>AAMIZTZKYHNGZKKYTPFSZAEMTRRZBRLRAWMAKSBIDAVLFTSYHNINYYSGWLYCYFGRKYAZVIBZVKAVTISKGIDGGMPWRRSFGBNIVYTDWKRDNFYSAVKKLVKGAKZIGIEHDHVTLBHRRZLZKALPGTEFVDVGZPVMWZRVIKSSEEZBLIRZGARISDIGGAATAAAISAGVPEYEVAIATTBAMVRZIARBFPYVELMDTWIWFQSGINTDGAHNPVTBRVVZRGDILSLNCFPMIFGYYTALERTLFLZZVBDASLZIWZKNTAVHRRGLZLIKPGARCKDIASELNBMYRZWDLLRYRTFGYGHSFGVLBHYYGREAGVELREDIZTVLEPGMVVSMEPMVMBPEGEPGAGGYREHDILV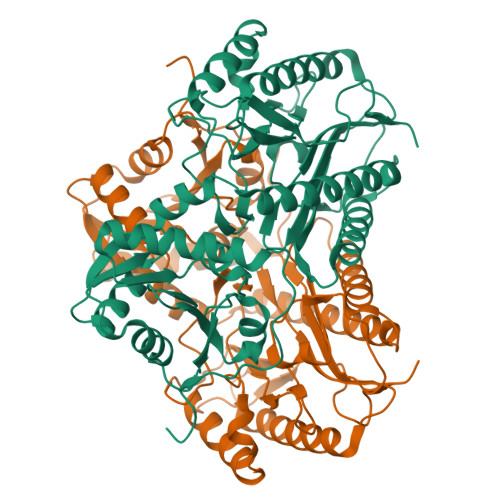IKENBTENITGFPFGPEHNIIKA[2x]>GMQEMEDLLYRLKVADETISNLFEKQLGISLTRYSILQTLLKDAPLHQLALQERL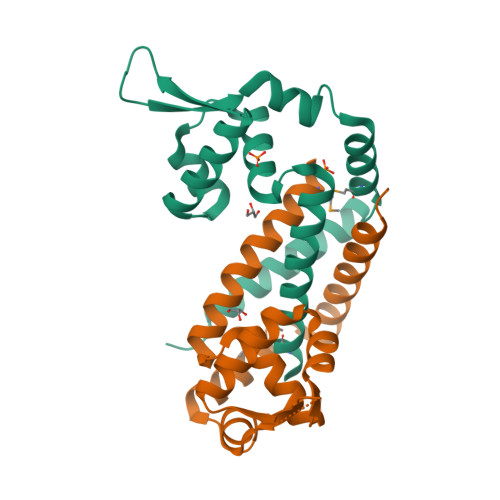QIDRAAVTRHLKLLEESGYIIRKRNPDNQREVLVWPTEQAREALITNPSAHHQAIKTSMNQILTVEESEQFLATLDKLLIGLQNLPI[4x]>[8x]EERPLVFLCSGCRRPLGDSLSWVASQEDTNCILLRCVSCNVSVDKEQKLSKREKENGCVLETLCCAGCSLNLGYVYRCTPKNLDYKRDLFCLSVEAIESYVLGSSEKQIVSEDK

To preserve centromere identity, CENP-A levels must be maintained through active CENP-A loading during the cell cycle. A central player mediating this process is the Mis18 complex (Mis18α, Mis18ý and Mis18BP1), which recruits the CENP-A specific chaperone HJURP to centromeres for CENP-A deposition. The Mis18 proteins, Mis18α and Mis18ý, possess a well-conserved globular domain called the Yippee domain (also known as the MeDiY domain; spanning residues 77-180 in Mis18α and 73-176 in Mis18ý) and C-terminal α-helices (residues 196-233 in Mis18α and 191-229 in Mis18ý). Here, using a multi-pronged approach, we characterise the structure of the Mis18 complex and show that multiple hetero- and homo-oligomeric interfaces facilitate the hetero-octameric Mis18 complex assembly composed of 4 Mis18α, 2 Mis18ý and 2 Mis18BP1.

To determine the structure of human Mis18 Yippee domains, we purified and crystalised Mis18α_Yippee_ (residues 77-190). The crystals diffracted X-rays to about 3 Å resolution, and the structure was determined using the molecular replacement method. The overall fold of the Mis18α_Yippee_ is remarkably similar to the previously determined *S. pombe* Mis18_Yippee_ homo-dimer structure. In brief, the monomeric Mis18α_Yippee_ is formed by two antiparallel ý-sheets that are held together by a Zn^2+^ ion coordinated via loops containing C-X-X-C motifs. The Mis18α_Yippee_ dimerisation is mediated via a back-to-back arrangement of a ‘three-stranded’ ý-sheet from each monomer. As observed for Mis18α_Yippee_ homo-dimer, the Mis18α/ý Yippee hetero-dimerisation is also mediated via the back-to-back arrangement of the three-stranded beta sheets of Mis18α and Mis18ý Yippee domains. The integrative model of the Mis18 complex fits well in the EM map. Interestingly, the serial arrangement of the Yippee domains utilises the second Yippee dimerisation interface observed in the crystal packing of both human Mis18α Yippee and *S. pombe* Mis18 Yippee (**Fig. S3d, highlighted by zoom in view**).>[2x]MKIYDTEGFPNPLRVRIALAEKGAT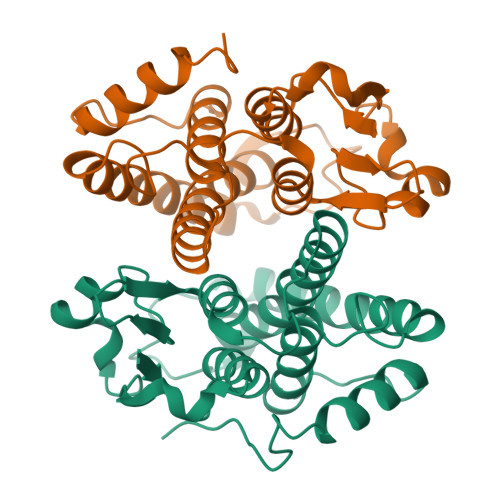DKVVFVPVDVMGGEHRTTDFRAKNPDATVPVLELDDGTCIAQCNAITEYLDGVFDGPSLTGASPKERAVIAMMNIRAESGLMNAVGAYFHHATRGLGPDLETWQCPDWGNKQKEVAQSTMAYLNEVLAENEFLAGDRFTVADITAYAGLVFAEFAKVDIPGHLDHLLAWRARVAARPSITGAENLYFQGHHHHHHHHHH> MSIVTKSIVNADAEARYLSPGELDRIKGFVTSGE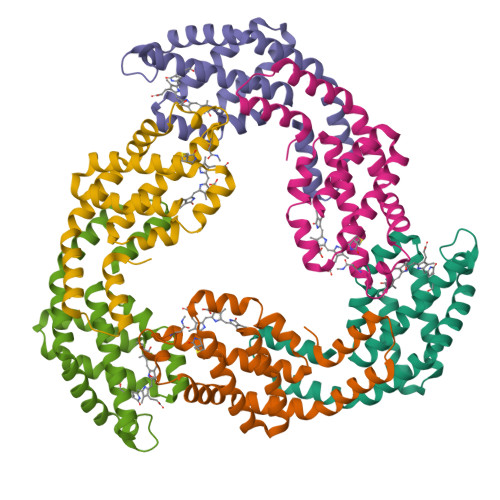RRLRIAQVLTESRERIVKQAGDQLFQKRPDVVSPGGNAYGEEMTATCLRDMDYYLRLITYGVVAGDVTPIEEIGLVGVREMYNSLGTPIPAVAEAVRCMKSVASSLLSGEDAAEAASYFDYVVGAMQ;> MQDAITAVINSSDVQGKYLDGSAMEKLKAYFQTGELRVRAATTISANAAEIVKDAVAKSLLYSDITRPGGNMYTTRRYAACIRDLDYYLRYSTYAMLAGDPSILDERVLNGLKETYNSLGVPVGATVQAIQAMKEVTATLVGADAGKEMGVYFDYICSGLS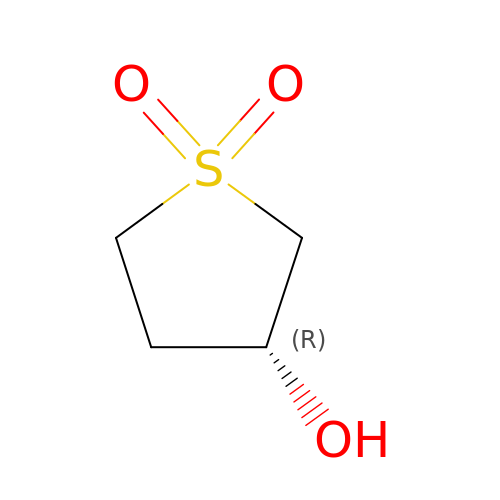3-hydroxythietane-1,1-dioxide | C4 H8 O3 S | AMXKVIWWXBYXRS-SCSAIBSYSA-N>MAHHHHHHVDDDDKMAQGLKDAYKDYFKIGVAVNNRNVADPDQIKVVLREFNSITAENAMKPQPTEPKKGEFNWEDADKIADFCRANGIKMRGHTLMWHSQIGSWMYQDEKGNLLSKEEFYANMKHHIQAIVNRYKDVVYCWDVVNEAVADSPVYPGRPEL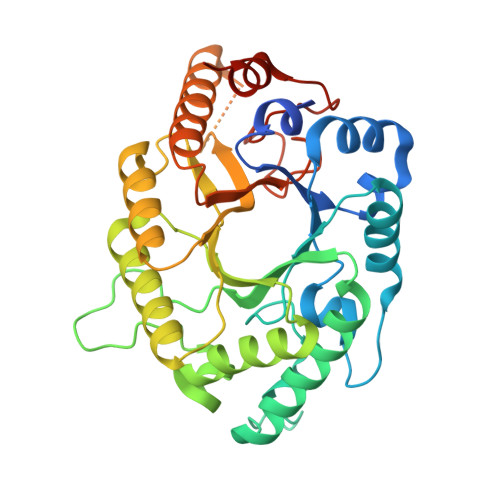RNSPMYQIAGEEFIYKAFEYAHEADPDALLFYNDYNDAEPAKSQRIYNLVKRMKDAGVPIDGIGMQAHYNVYGPTMKEVDDAIKLYSTVVDHIHLTELDIRINEDMGGGLRFNQGQATVSDWERTLQQDQYVQLFKVLRKHKDVIDCVTFWNVSDKDSWLGVRNYPLLFDENYKPKQAYNAVKNFDPKMDNAVI[2x]1~{H}-1,2,3-triazole | C2 H3 N3 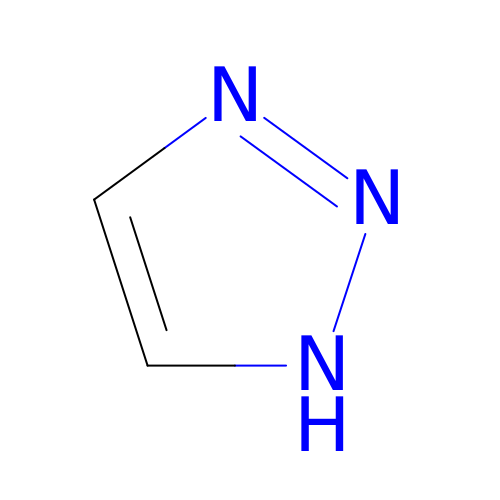| QWENRTYMTSOGBR-UHFFFAOYSA-N>[2x]EFLGDGGDVSFSTR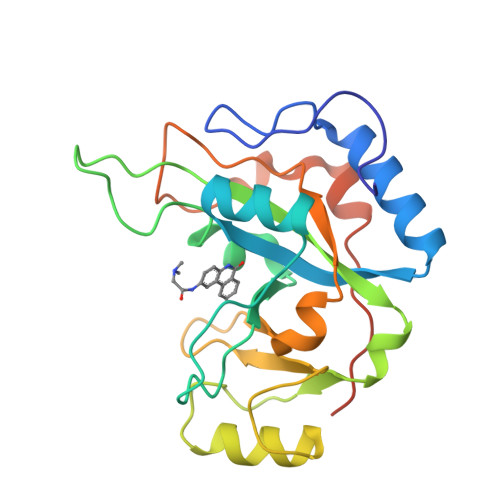GTQNWTVERLLQAHRQLEERGYVFVGYHGTFLEAAQSIVFGGVRARSQDLDAIWRGFYIAGDPALAYGYAQDQEPDARGRIRNGALLRVYVPRSSLPGFYRTSLTLAAPEAAGEVERLIGHPLPLRLDAITGPEEEGGRLETILGWPLAERTVVIPSAIPTDPRNVGGDLDPSSIPDKEQAISALPDYASQPGKPPREDLK> 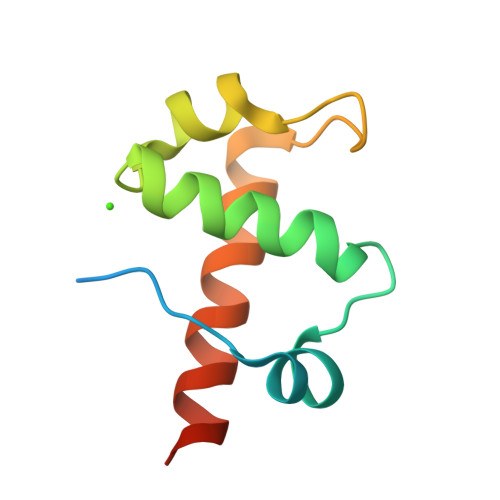GGKDYPFARFNKTVQVPVYSEQEYQLYLHDDAWTKAETDHLFDLSRRFDLRFVVIHDRYDHQQFKKRSVEDLKERYYHICAKLANVRAVPGTD>MMNFTLLTYLADCQPKVRSELEKFSKNLEEDIQQLREIGLDILVDGQDYRLVPMLPLLNPQQISTALFPYSIHYQPIISSTNEWILQNILSLKKGDLCVAEYQTAGRGRRGRQWLSPFAGQIMFSFYWAFDPKKSIEGLSLVIGLAIAEVLNVQVKWPNDILFDERKLGGILVEIANHKNGMLNLVIGIGINVSLSKQTEISQPYAEVCEIDPDVERQTLLPKLIQHLYTRLNIF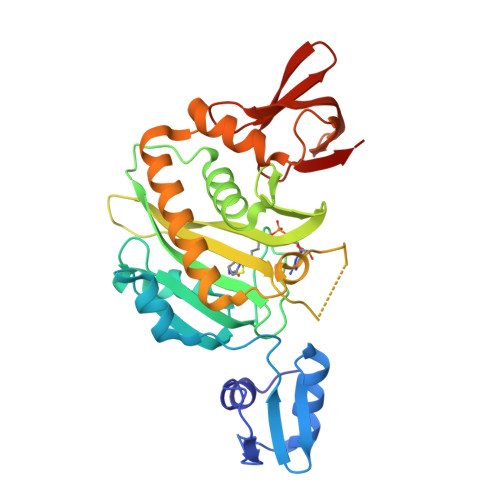EQNGIDEEFQQAWQSYNAFSNSEINVLTEQGVISGIEQGIDERGYLKVLCGNKIQMFNGGEVSLRKK[2x]> ENY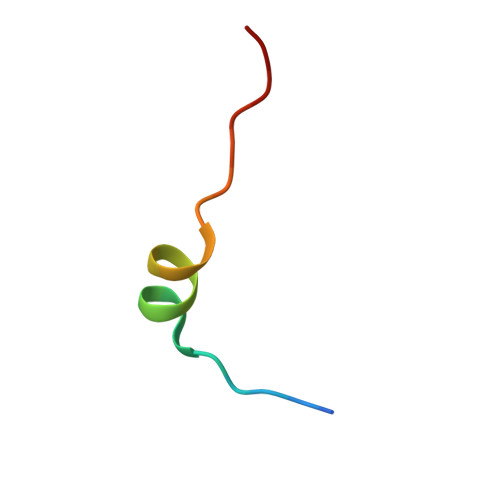SNTDPEELLRKHVFPSVPK5-nitrosalicylic 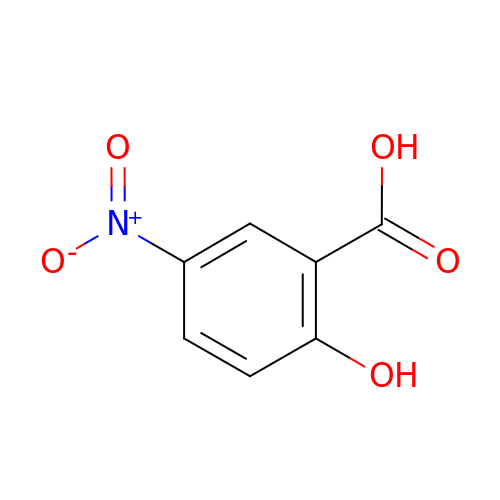acid | C7 H5 N O5 | PPDRLQLKHRZIJC-UHFFFAOYSA-N>[2x]MNIVLMGLPGAGKGTQAERIVAKYGIPHISTGDMFRAAMKEETPLGLEAKSYIDKGELVPDEVTIGIVRERLSKSDCERGFLLDGFPRTVAQAEALEEILEEMGRKLEYVIHIEV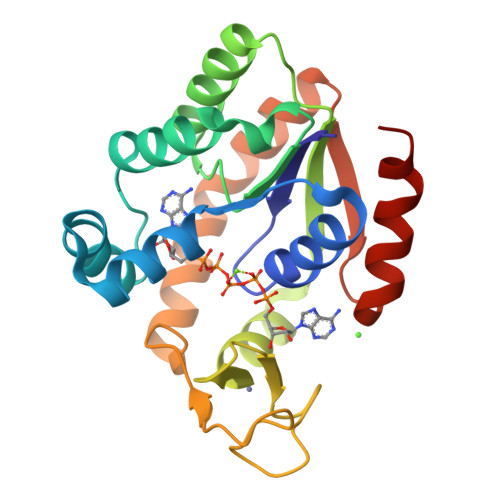RQEELMERLTGRRICSVCGTTYHLVFNPPKTPGICDKDGGELYQRADDNEETVAKRLEVNMKQMAPLLAFYDSKEVLVNVNGQQDMEKVFKDLREILQGLAR>MADSGYLFSVRGRVACVTGASSGLGRRAATVLAQAGAQVVGVARRADALAEWQAEAGGETHAIPYDLSDRDGLEGLARQVVDPFGAPDILVHAAGINTRQPADEVTPEGWDITLTLNLSVPFFLSQYLVPGMKARGWGRIVNFASLQTTRAFPGGIAYGASKGGVAQMTRAMAEAWSPHGITANALGPGFFRTELTAPVFADPERAARNAAQTCIGRNGEPEDLDGPLLFLCSQASAYVTGQVLMVDGGYTAK[4x]

Dihydroxypropanesulfonate (DHPS), a globally abundant organosulfur compound, serves as an ecologically important currency for nutrient and energy transfer from phytoplankton to bacteria in the ocean. A novel chiral-selective DHPS catabolic pathway was identified in marine Roseobacteraceae strains, where HpsO and HpsP dehydrogenases at the gateway to DHPS catabolism act specifically on R-DHPS and S-DHPS, respectively. R-DHPS is also a substrate for the dehydrogenase HpsN. All three dehydrogenases generate stable hydrogen bonds between the chirality-center hydroxyls of DHPS and highly conserved residues, and HpsP also form coordinate–covalent bonds between the chirality-center hydroxyls and Zn2+, which determines the mechanistic basis of strict stereoselectivity.

The crystal structure of RpHpsO shows that it exists as a tetramer in the asymmetric unit, with seven-stranded parallel β-sheets sandwiched by six α-helices, constituting a typical Rossmann-fold domain in each monomer. RpHpsO is a member of the short chain dehydrogenase/reductase (SDR) family, which has two defining features, an N-terminal domain responsible for coenzyme NAD(H) or NADP(H) binding and a C-terminal domain harboring the essential catalytic residues. The results showed that the orientation of the C3-OH of R-DHPS was toward the reactive center (C4) of the nicotinamide ring of NAD+ with a distance of ~3 Å, which was appropriate for hydride transfer. Ser145 and Tyr158 both formed hydrogen-bonding interactions with the C3-OH of R-DHPS. The Ser, Tyr, and Lys residues are conserved in other SDR family enzymes and constitute a catalytic triad, suggesting their essential role in RpHpsO catalyzation of R-DHPS. However, enzymatic activity of the Leu116Ala mutant for R-DHPS did not decline significantly. This demonstrated that Ser145, Tyr158, and Lys162 function as catalytic residues in RpHpsO. Gln147 formed a hydrogen bond with the chirality-center hydroxy (C2-OH) of R-DHPS, suggesting that Gln147 may have a vital role in specific recognition of R-DHPS. Mutant Gln147Ala abolished the most enzymatic activity of RpHpsO for R-DHPS. These results demonstrated that the interaction between Gln147 of RpHpsO and C2-OH of R-DHPS appears to drive the specificity of RpHpsO for the R-DHPS enantiomer.>MRIQHNIAALNTHRNLAANNAAASKNLEKLSSGFKINRAGDDAAGLAISEKMRGQISGLNMASKNSSDAISLIQTAEGGLNETHAILQRMRELAVQSRNDTNDEATNDRSNLNDELKQLQEEITRISSQMEFNNKKLLDGSQSTNGLTFQIGANAGQTITMKISTMSATKLGVDAAKASISKGTAASKAIKSIDDAINTVSKTRSALGAVQNRLEHTINNLGTSAENLTAAESRIRDTDMAAEMMAFTKNNILTQAAQSMLAQANQQPQGVLQLLQ[44x]

The flagellar filament is composed of the protein flagellin that assembles into linear protofilaments. The 11 flagellar protofilaments twist into a supercoil that can vary in rise and handedness, a phenomenon termed polymorphism. Each protofilament can exist in the so-called L- or R-state, depending on the conformation of its composing flagellin monomers. Kurthia is a Gram-positive bacterium belonging to the Firmicute phylum.

We analyzed wild-type, mostly curved flagellar filaments projecting from motile Kurthia bacteria by transmission cryo-electron microscopy. Helical reconstruction resulted in a map with a maximum resolution of 2.6 Å or better of the most ordered parts and an overall resolution of 2.8 Å (EMD-10362). A comparison of the 3D structure of flagellin from Kurthia (276 amino acids) and the published structures of L- and R-conformations of B. subtilis (304 amino acids) show that all share the same overall fold, including five helices and two β-hairpins, but that the loops before and after the β-hairpins were shorter in Kurthia. Kurthia flagellin was present in a conformation that was most like the L-state as encountered in B. subtilis. Initially, five 3D classes were identified, which upon helical refinement (including the refinement of the helical parameters) produced good quality potential maps that were so similar that combining the five classes significantly increased the resolution. This suggested that flagellin was essentially present in a single conformation, in which the 11 protofilaments were tilted slightly left by ~ 0.06°. The electron scattering potential map of the functional Kurthia filament showed six extra densities corresponding to O-glycosylations of threonines and serines. Our data indicate that wild-type Kurthia flagellin was present in just one single conformation, and formed nearly parallel protofilaments, irrespective of flagellar curvature. This suggests that in Kurthia, the polymorphic switching of the flagellar supercoil from left- to right-handed and vice versa, as induced by reversal of the flagellar motor, might not require a conformational change of the flagellin monomers.> MPMTVITLKNVPQSLRGDLTRWMQEIATGVYVGNFNSRIREYLWRRVQETMGAGEASMCFAARNELGYDFLTENASRSVIDYDGLPLIFIPKEQSAVSDLPKGFSTAAKLHRAHIAGSGKKKEKPIRYVVIDIETDGKDAKRNHILEIGAIRCEDGKETHFTAL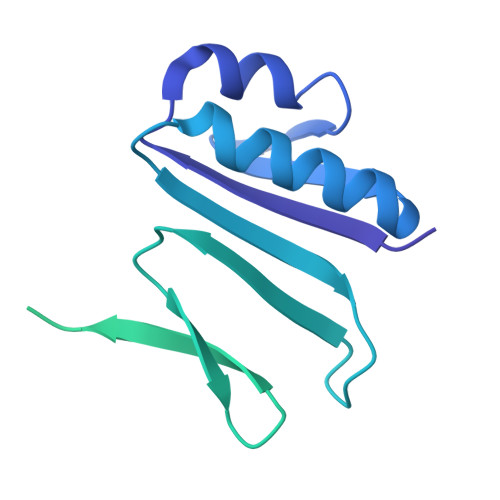ISGDAVPPSITKLTGITATLLQKEGQEEKKVLTAFREFIGDDDLVGYHVSFDIEFLRQAFKKYGLGYLKNKTHDLLRIVKKEQLFQADYKLETSLQSYGIHKKVPHRALGDAELVKCLAKKLNKF(2~{S})-2-[bis(pyridin-2-ylmethyl)amino]-5-(3-phenyl-5-sulfanylidene-1~{H}-1,2,4-triazol-4-yl)pentanoic 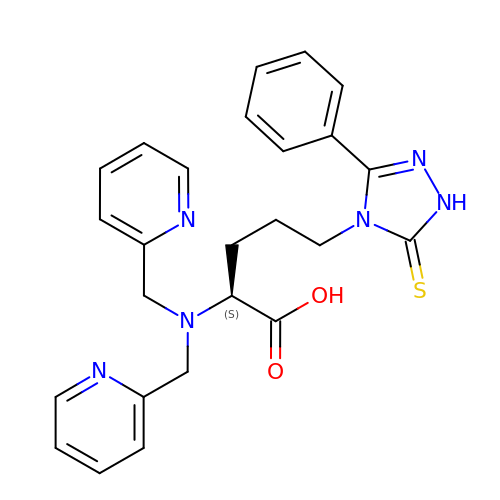acid | C25 H26 N6 O2 S | DXFIRCHAKLZTEP-QFIPXVFZSA-N> DPERPALGILELSSYARGVKVADAALKAAPVK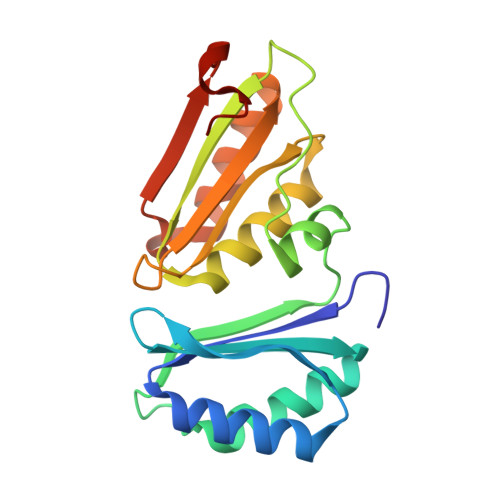LLKCEPVEPGRALIMLLGEPEDVAKAMIAALDVAGLGSGNLIDYALIPEIHPQLLPFLKEYKKSEPIKDPNKAIIVAEVSTVAAAIEAADVALRLANVELTSMRLAEHIGGRASFTLIGDKEDVEKAARAIRGVAGERLLDLEIIEKPVEALIGNEFF[2-(1-heptyl-1H-imidazol-3-ium-3-yl)ethane-1,1-diyl]bis(phosphonate) 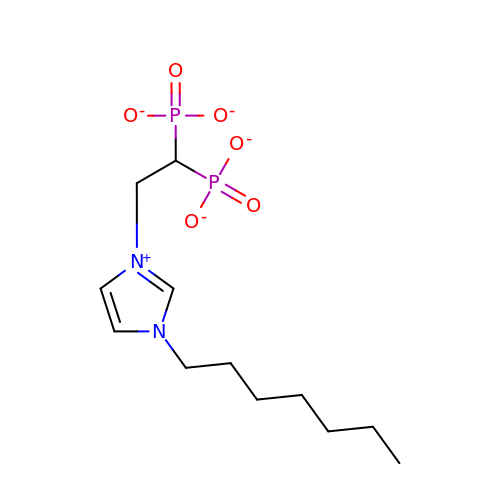| C12 H21 N2 O6 P2 | GQXQNORVSDKRHM-UHFFFAOYSA-K> UGCUCCUAGUACGA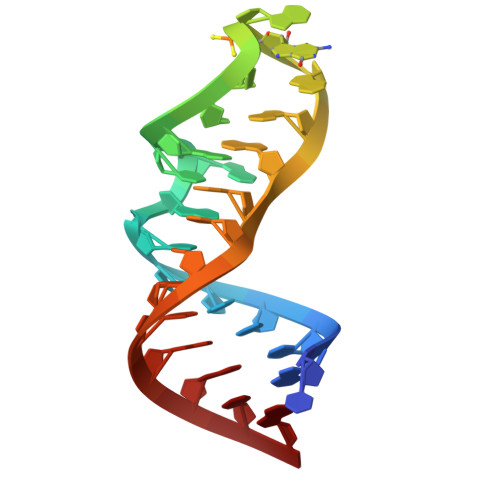XAGGACCGGAGUG>[2x]GMLIPPSTFLPKRDKNVPYIAEVQSIPLSPSAYSVIIKDKSIFETSLSPNGSVSMSSFLTSIFDSAYIASLKYKSDDNYKYIGIPLLNAFVEWQIEEIDDSLDDKSKEIIKSYLISKLSAKYEKTKTENAVRVRLSICRDLYDTLSSDDLYYENKVYSLTLRRFLKAVYEDYALLSDCERERLI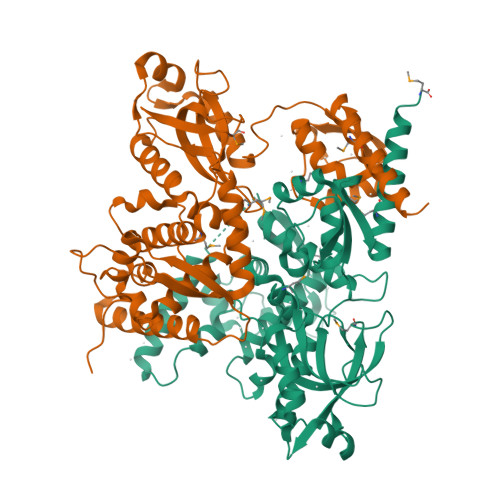FADNIIKINEVIKQNGSRYYSFIYAYSNMYSREKRRIRLIPYRIVSDEYKMYNYLVCLSDEKSAGKEFKADSYRISRLSGLSIAEKLSQKEYSSVTEYERLKEGHVKSVKHLLSDPRFGSDESDISKVYLTEKGVEMFRKILYQRPILKGNEKPKPNTVNEFISPPIQVKYYFNKFGKDGVILSPSDSFEEMRTLYVEGADAYNREVEM> SQATEYVLRSVIAKEVGDILRV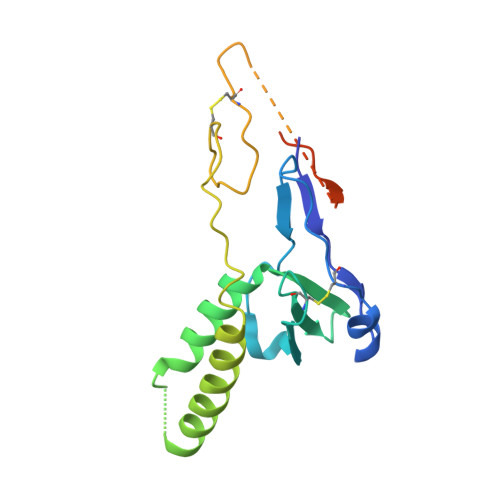PCMRTPADDVSWRYEAPSVIDYARIDGIFLRYHCPGLDTFLWDRHAQRAYLVNPFLFAAGFLEDLSHSVFPADTQETTTRRALYKEIRDALGSRKQAVSHAPVRAGCVNFDYSRTRRCVGRRDLRPANTTSTWEPPVSSDDEASSQSKPLATQPPVLALSNAPPRRVSPTRGRRRHTRLRRN> QDFRKYEEGFDPYSMFTPEQIMGKDVRLLRIKKEGSLDLALEGGVDSPIGKVVVSAVYERGAAERHGGIVKGDEIMAINGKIVTDYTLAEAEAALQKAWNQGGDWIDLVVAVCPPKEYDD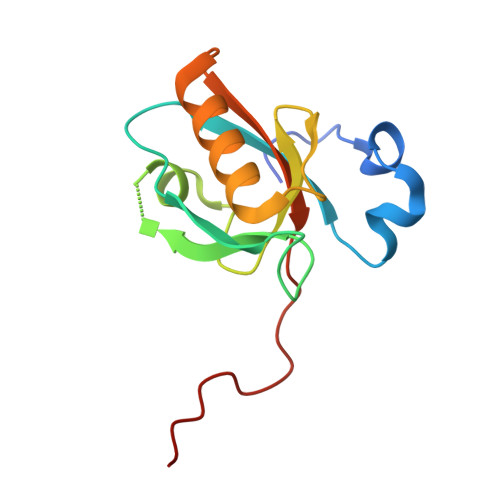ELTFF In this paper, we report the crystal structures of a lectin from Agrocybe aegerita, designated as AAL2, in its apo- and complex forms with GlcNAc and GlcNAcβ1-3Galβ1-4GlcNAc, as part of our endeavors to develop a system to facilitate the identification and purification of O-GlcNAcylated proteins. AAL2 was recently discovered from the fruit body of the edible mushroom A. aegerita. AAL2 was found to specifically bind nonreducing terminal N-acetylglucosamine (GlcNAc) moieties of either alpha- or beta-linkage and was reported to have the activity of inducing apoptosis in hepatoma cells in vitro as well as inhibiting hepatoma growth in tumour-bearing mice in vivo. The overall structure of AAL2 monomer is a single domain with the shape of cylindrical torus with a diameter of about 51Å and a height of about 27Å, showing a very regular, seven-bladed β-propeller fold formed by the blades packing in a circular array.

The structures of AAL2, AAL2-GlcNAc and AAL2-GlcNAcβ1-3Galβ1-4GlcNAc were determined at resolutions of 2.0Å, 2.1Å, and 2.0Å, respectively. There are two virtually identical AAL2 monomers arranged around a two-fold pseudoaxis of symmetry in an asymmetric unit in both the structures of AAL2 and AAL2-GlcNAc, and one AAL2 monomer in AAL2-GlcNAcβ1-3Galβ1-4GlcNAc, while the protein exists as monomers in solution as determined from its elution volume on a Superdex 200 10/300 GL column. As expected from the sequence homology, the structures of AAL2 and AAL2-GlcNAc complex are very similar to those of the corresponding structures of PVL, with root-mean-square deviations (RMSDs) of 0.7Å for Cα atoms. Each blade is a β-sheet consisting of four anti-parallel β-strands arranged in a W-like shape and of about 56 residues in length, and is named W-motif according to its shape. Seven tandem W-motifs of the AAL2 monomer, numbered WI to WVII from N- to C-terminus, are organized around a seven-fold axis of pseudo symmetry. The first β-strands of the seven W-motifs are located innermost of the AAL2 monomer and form a central tunnel that is filled with water molecules and almost blocked by a long N-terminus loop (except for a small opening). These 7 innermost strands point to the same direction, from the ‘entrance’ to the ‘exit’ of the central tunnel, and run almost parallel to each other along the direction of the seven-fold propeller axis. What is notable is that the seven sequence repeats observed in AAL2 do not match exactly with the seven blades, but instead have a shifting of one β-strand. WI consists of three consecutive strands, i.e., strands 2, 3 and 4 at the N-terminus, and one strand, i.e., strand 1, from the C-terminus.

>[2x]TSNVITQDLPIPVASRGFADIVGFGLDGVVIGRNAVNLQPFLAVKNFAQNAGGWLTTKHVRLIADTTGTGKGDIVGFGNAGVYVSVNNGKNTFADPPKMVIANFGYDAGGWRVEKHLRYLADIRKTGRADIIGFGEKGVLVSRNNGGLNFGPATLVLKDFGYDAGGWRLDRHLRFLADVTGNGHLDIVGFGDKHVFISRNNGDGTFAPAKSVIDNFCIDAGGWKIGDHPRFVADLTGDGTADIIGCGKAGCWVALNNGGGVFGQVKLVINDFGTDKGWQAAKHPRFIADLTGNGRGDVVGFGNAGVYVALNNGDGTFQSAKLVLKDFGVQQGWTVSKHRRFVVDLTGDGCADIIGFGEKETLVSYNDGKGNFGPVKALTNDFSFSGGKWAPETTVCWMANLDSSRH>[2x]SLRSDLINALYDENQKYDVCGIISAEGKIYPLGSDTKVLSTIFELFSRPIINKIAEKHGYIVEEPKQQNHYPDFTLYKPSEPNKKIAIDIKTTYTNKENEKIKFTLGGYTSFIRNNTKNIV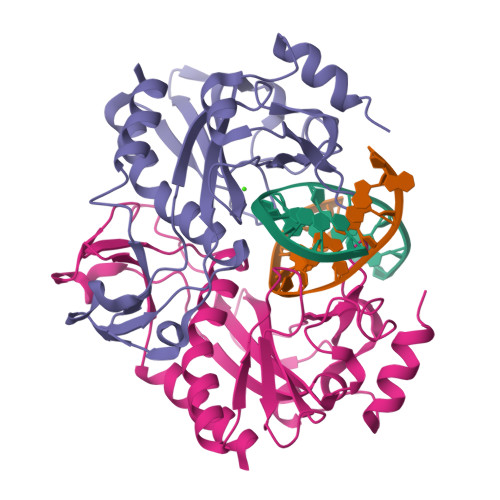YPFDQYIAHWIIGYVYTRVATRKSSLKTYNINELNEIPKPYKGVKVFLQDKWVIAGDLAGSGNTTNIGSIHAHYKDFVEGKGIFDSEDEFLDYWRNYE N-(5-{[(5S)-7-(5-methylimidazo[1,2-a]pyrimidin-7-yl)-2,7-diazaspiro[4.4]nonan-2-yl]methyl}-1,3-thiazol-2-yl)acetamide 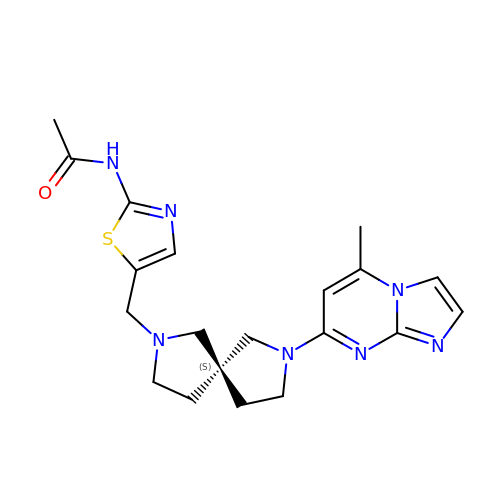| C20 H25 N7 O S | RJDUUKXZMXIWIE-FQEVSTJZSA-N>[6x]MENSEKTEVVLLACGSFNPITNMHLRLFELAKDYMNGTGRYTVVKGIISPVGDAYKKKGLIPAYHRVIMAELATKNSKWVEVDTWESLQKEWKETLKVLRHHQEKLEASDCDHQQNSPTLERPGRKRKWTETQDSSQKKSLEPKTKAVPKVKLLCGADLLESFAVPNLWKSEDITQIVANYGLICVTRAGNDAQKFIYESDVLWKHRSNIHVVNEWI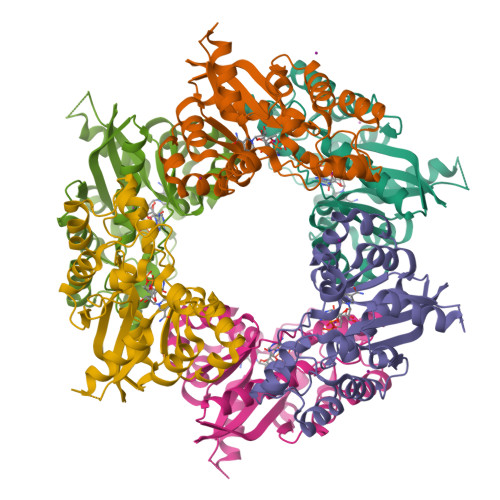ANDISSTKIRRALRRGQSIRYLVPDLVQEYIEKHNLYSSESEDRNAGVILAPLQRNTAEAKT>MVKPEEVDKAYEVAKQRYAEIGVDTDAAMKELEKVPLSVHCWQGDDIHGFLFPNQELTGGIGVSGNYPGIARTPDELAGDMHEALSLIPGKHRVQLHAIYAVTDKKRDLDTLEPEDFDYWIDWAKQEGVGLDFNGTFFSHPMVKDNMTVSSPDPKVRDFWIRHGKISREISNYIGEKLGSQVVNNFWLPDGFKDNPIDKKTPRLRLLKALDEIIKDPLPEKNTIESFEGKLFGTGIESYTTGSHEFYQNYAISRNKLWTIDAGHFHPTEDVSDKFSAFFPFGKGLFMHVSRPVRWDSDHVVIMDDALIRITRSLVRDGYLDRTHIGLDFFDATINRVAAWVVGARATQKSLLQAMLAPIDQLKKDELNADFTTRLIETEELKSFPFGAVWDKFCQDHNTPVGFDWMNNIHQYEKDVQFKRDAKLVHGSHHHHHH[4x]

L-RhI is one of the enzymes involved in L-rhamnose metabolism and catalyzes the reversible isomerization between L-rhamnose and L-rhamnulose. Herein, we report the crystal structures of L. rhamnosus Probio-M9 L-RhI (LrL-RhI) in complexes with L-rhamnose, D-allulose, and D-allose, which show enzyme activity toward L-rhamnose, D-allulose, and D-allose in acidic conditions, though the activity toward D-allose was low. All structures belong to the orthorhombic space group P212121 with four molecules (Mol-A, Mol-B, Mol-C, and Mol-D) forming a homotetramer in an asymmetric unit. The overall structure of LrL-RhI is similar to the known structures of L-RhIs.

In the complex with D-allulose, D-allulofuranose and ring-opened D-allulose were observed in the catalytic site. The bound D-allulose shows a ring-opened structure. The catalytic metal likely moves between two positions (Mn2A and Mn2B) and is refined as alternative metals Mn2A and Mn2B with 0.8 and 0.2 occupancies, respectively, considering the electron density maps and b-factors. The catalytic metal at the position of Mn2B can be coordinated by His264 and Asp296, two water molecules (W4 and W6), and O1 and O2 of D-allulose. O1 and O5 of D-allulose are recognized by Lys230 and His97, respectively, and Trp187 faces the hydrophobic side of D-allulose. In addition, Leu57 and Ile61 on the flexible loop region cover the active site and create a hydrophobic environment along with Phe138, Ile47, and Phe330 orienting to D-allulose. In the structure of LrL-RhI/D-allulose, an alternative conformation of D-allulose was found, α-D-allulofuranose (before ring-opening, yellow stick model) and ring-opened D-allulose (yellow line model). His97 recognizes O4 of α-D-allulofuranose instead of O5 of D-allulose. In this study, the flexible loop region of LrL-RhI was observed in the LrL-RhI/D-allulose complex; however, the corresponding regions in most of the LrL-RhI structures are also missing, suggesting that these regions are highly flexible.>[8x]MNNNKRSKLSTVPSSRPIRVGFVGLTSGKSWVAKTHFLAIQQLSSQFQIVALYNPTLKSSLQTIEQLQLKHATGFDSLESFAQYKDIDMIVVSVKVPEHYEVVKNILEHSSQNLNLRYLYVEWALAASVQQAEELYSISQQRANLQTIICLQGRKSPYIVRAKELISEGCIGDINSIEISG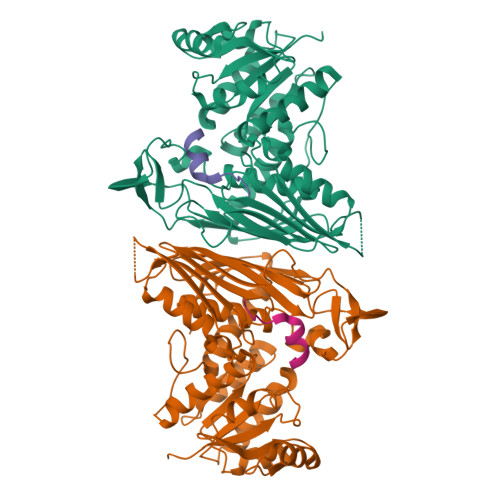NGGWYGYERPMRSPEYLYDIESGVNLISNSFGHTIDVLQYITGSYFQKINAMISNNIPTQFLLDENGKRTKETISKTCPDHLLFQGILENGKVPVSCSFKGGTPVKKLTKNLVIDIHGTKGDLKIEGDAGFVEISNLVLYFYGIKNGNGSSNGTDNNGAAAIKDKEKVTKSPSPSTGTSEEEQTMEVFHLRNYNSVVGNILRIYESIADYHFLGKPESKSSRGPDDLFASTKFDKQGFRFEGFPTFKDAIILHRLIDAVFRSDKEEKTLDVSKIMILEHHHHHH;>TQQLFNTTTMDDVYNYIFDNDE[8x]> EEDLTEVKKDALENLRVYLCEKIIAERHFDHLRAKKILSREDTEEISCRTSSRKRAGKLLDYLQENPKGLDTLVESIRREKTQNFLIQKIT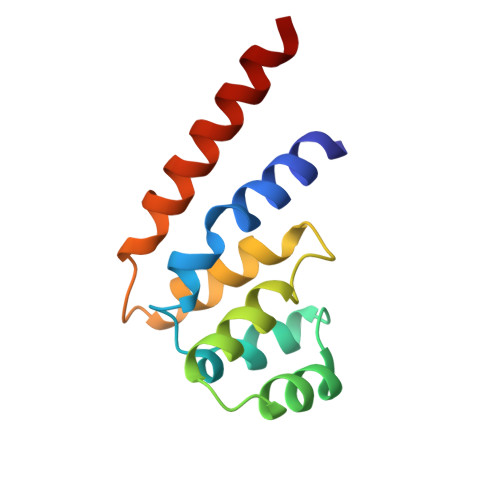DEVLKLRNIKLEHLK Fluorescent proteins have facilitated major breakthroughs in modern molecular cell biology. They are widely used for studying biological events, such as cellular trafficking and endocytosis, and have contributed to the development of innovations such as multiphoton microscopy, genetically-encoded sensors, and super-resolution microscopy. mKate, a derivative of eqFP578 from Entacmaea quadricolor, is a bright, monomeric, far-red fluorescent protein with excitation and emission peaks at 588 nm and 635 nm, respectively. Structural characterization of mKate under different conditions revealed the pH-dependent trans-cis isomerization of its chromophore, a discovery that further aided the development of mKate variants with enhanced optical properties. Using a structure-informed approach, we introduced a minimal set of two mutations in the chromophore environment of mKate. The first mutation, S158A, has been shown to destabilize the trans conformation of the chromophore, whereas the second mutation, S143C, was intended to impact the cis conformation.

Mutation S143C may de-stabilize the cis-conformation by removing a hydrogen bond between the side chain of S143 and the chromophore. The chromophore in the crystal structure of mKateS143C adopts only the trans-conformation at neutral pH, consistent with the proposed role of S143 in stabilizing the cis-conformation and the spectral properties of the protein. The brightness of the single-mutant mKateS143C is more than 100-fold less than that of mKateS158A, consistent with a destabilization of the cis-chromophore, which was predicted for this mutation based on the mKate crystal structure.

>AAASMSALITENMHMKLYMEGTVNNHHFKCTSEGEGKPYEGTQTMRIKVVEGGPLPFAFDILATSFMYGSKTFINHTQGIPDFFKQSFPEGFTWERVTTYEDGGVLTATQDTSLQDGCLIYNVKIRGVNFPSNGPVMQKKTLGWEACTEMLYPADGGLEGRSDMALKLVGGGHLICNLKTTYRSKKPAKNLKMPGVYYVDRRLERIKEADKETYVEQHEVAVARYCDLPSKLAHK[4x]> FARSLSITTPEEMIEKAKGETAYLPCKFTLSPEDQGPLDIEWLISPADNQKVDQVIILY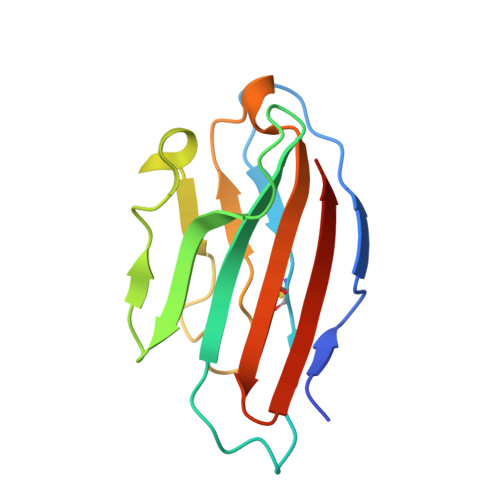SGDKIYDDYYPDLKGRVHFTSNDLKSGDASINVTNLQLSDIGTYQCKVKKAPGVANKKIHLVVLV As the main entry gate of mitochondria, the TOM complex is responsible for transferring ~90% of mitochondrial proteins from the cytosol into the mitochondria. Mitochondrial proteins are primarily synthesized within the cytosolic ribosome and subsequently transferred to specific mitochondrial compartments through the corresponding translocase complexes, including the translocase of the outer mitochondrial membrane (TOM) and the translocase of the inner mitochondrial membrane (TIM23). The TOM complex consisted of two Tom40 pores, which were surrounded by two copies of three small Tom subunits and tethered by two Tom22 molecules. To investigate the transfer process of preproteins from cytosol to the mitochondrial matrix, we captured the TOM–TIM23 supercomplex by translocating Jac1sfGFP to isolated yeast mitochondria to obtain TOM–TIM23–Jac1sfGFP supercomplex.

Notably, the density of the TIM23 complex was progressively diminished with the contour level value increasing from 0.08 to 0.16, implying the instability of the TIM23 complex. Numerous efforts were made including substrate screening and modification, large-scale image collection, and chemical crosslinking to enhance stability of the TIM23 complex to generate a high-resolution map, but no obvious improvements were achieved for the TIM23 map. In the architecture of the TOM–TIM23–Jac1sfGFP supercomplex, the structural features of the TOM complex were significantly clearer than those of the TIM23 complex. The densities corresponding to Jac1 polypeptides and sfGFP were observed within the Tom40 channel and on the cytosolic side of the Tom40, respectively. Moreover, structural analysis of the Jac1sfGFP-engaged TOM complex revealed two preproteins proximity sites (PPS) on the mitochondrial surface. The PPS1 corresponded to the N-terminus of Tom5 (residues 1–26), while the PPS2 encompassed the loop between β-strands 14 and 15 of Tom40. The PPS1 and PPS2 were situated on the cytosolic side of the TOM complex, potentially functioning in recognizing the incoming preproteins. Superposition analysis of the free TOM complex and Jac1sfGFP-engaged TOM complex showed that Tom5 exhibited an ~3-Å movement towards the Tom40 channel in the Jac1sfGFP-engaged TOM complex, suggesting that the Tom5 might respond to the incoming substrates.

>[2x]MVELTEIKDDVVQLDEPQFSRNQAIVEEKASATNNDVVDDEDDSDSDFEDEFDENETLLDRIVALKDIVPPGKRQTISNFFGFTSSFVRNAFTKSGNLAWTLTTTALLLGVPLSLSILAEQQLIEMEKTFDLQSDANNILAQGEKDAAATAN;>MFGLPQQEVSEEEKRAHQEQTEKTLKQAAYVAAFLWVSPMIWHLVKKQWK[2x];>MDGMFAMPGAAAGAASPQQPKSRFQAFKESPLYTIALNGAFFVAGVAFIQSPLMDMLAPQL[2x];>[2x]MSFLPSFILSDESKERISKILTLTHNVAHYGWIPFVLYLGWAHTSNRPNFLNLLSPLPSV;>MSAPTPLAEASQIPTIPALSPLTAKQSKGNFFSSNPISSFVVDTYKQLHSHRQSLELVNPGTVENLNKEVSRDVFLSQYFFTGLRADLNKAFSMNPAFQTSHTFSIGSQALPKYAFSALFANDNLFAQGNIDNDLSVSGRLNYGWDKKNISKVNLQISDGQPTMCQLEQDYQASDFSVNVKTLNPSFSEKGEFTGVAVASFLQSVTPQLALGLETLYSRTDGSAPGDAGVSYLTRYVSKKQDWIFSGQLQANGALIASLWRKVAQNVEAGIETTLQAGMVPITDPLMGTPIGIQPTVEGSTTIGAKYEYRQSVYRGTLDSNGKVACFLERKVLPTLSVLFCGEIDHFKNDTKIGCGLQFETAGNQELLMLQQGLDADGNPLQALPQL[2x]>[2x]MNLKPQTLMVAIQCVAARTRELDAQLQNDDPQNAAELEQLLVGYDLAADDLKNAYEQ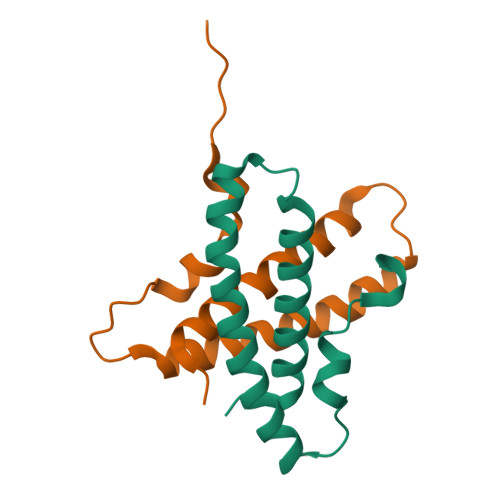ALGQYSGLPPYDRLIEEPASLEHHHHHH> MERLFEELAGEAVKELLRAVRGTFFCRSTAERLRRNVEPLLPLVQPQAAQGGGGWGHGRSAGELAELAAQLREALELARRAASAPRWNVYRTAQLARRMEAADTAIARWLSRHAPAHVLDGVRRLRDEADARIGRLERRVEEVAAAQQQQQAAATALPPPAISLPFALPPPPPPPKAMAMMAMDTPPTKGMAVGMEVELPFPDDEEDESMVGGGVRVGKEKVKEMVMSGGGGGWEAVGICGMGGSGKTTLAMEIFKDHKIRGYFSDRVFFETISQSANLDTIKMKLWEQISGNLVLGAYNQIPEWQLKLGPRDKGPVLVILDDVWSLSQLEELIFKFPGCKTLVVSRFKFPSLVTR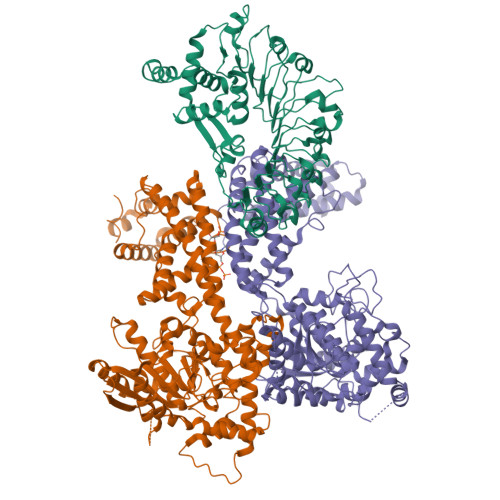TYEMELLDEEAALSVFCRAAFDQESVPRTADKKLVRQVAAECRGLPLALKVIGASLRDQPPKIWLSAKNRLSRGETISDSHETKLLERMAASIECLSGKVRECFLDLGCFPEDKKIPLDVLINIWMEIHDLDEPDAFAILVELSNKNLLTLVNDAQNKAGDLYSSYHDFSVTQHDVLRDLALHMSGRDALNNRRRLVMPRREESLPKDWQRNKDTPFEAQIVSIHTGEMKESDWFQMSFPKAEVLILNFASSVYYLPPFIATMQNLKALVLINYGTISATLDNLSAFTTLSDLRSLWLEKITLPPLPKTTIPLKNLRKISLVLCELTNSLRGSKVDLSMTFPRLSNLTIDHCIDLKELPSSICEISSLESISISNCHDLTELPYELGKLHCLSILRVYACPALWRLPPSVCSLKRLKYLDISQCVNLTDLPEELGHLTSLEKIDMRECSRLRSLPRSSSSLKSLGHVVCDEETALLWREAEQVIPDLRVQVAEECYNLDWLVD;> MPAAAALSDDDRLVVAHCAALSFPPASQPPPPPTTSSSSSGAGAGASFQVHHASHPYPCAAFAFPPSWSAAPGWAAAGRAAFGDAEVDPSLFPSLRSVGSGVPARANAAFLASFGALLDGSPLQSEVSRAVAEEKRIVFTGHSSGGSIATLAAIWFLETCTRRGSVNQAHPFCVTFGAPLVGDNTFNNAVRREGWSQCILNFVVPVDIIPRIPLTPLASATEGIQAVLDWLSPQTPNFSPSGMPLIISQFYENLLRSTLSIASYEACSFMGCTSSILGTLTSFIELSPYRPCGTYLFLTSSEQLAVLTNSDAVLQLLFYCLQLDPQQQLRDAAERSLSAHWQYEPIKQSMMQEIVCVDYLGVVSSTLPGRQMSSTIVGGLELSKEAMLSLSAAGQWEKQRETNQAKIDGASCTKIREALKSLNEYKRTCELHEVSYYDSFKLQREVHDFNANVSRLELAGLWDEIVEMLRRRELPDGFESRQDWVNLGTLYRRLVEPLDIANYYRHSKNEDTGSYLSKGRPRRYKYTQEWHEQSQRISFGSSLESCFWAMAEELQAEIANGKTFEDVRDRVVKLESDAHGWSMSGSLGKDIFLSRSSFVIWWKTLPENHRSASCIAKLVPW;> MEDASRGEEENSMFETSHVLGALLASSPLLARAWDRCAAAADGGASSLGFVHGGGGGGEGEPVCVAFSGVQAALSAAAGGGGGAEIFKPVGLRGDAAGRLFAPLVAAEPEDAGGEPVAVQALALQGFLRLCRSPEFQVLLNQIRGKAVVFTGHSLGGAIAALVALHYLCTSSSSSAFAPAPPVLCVTFGSPLLGNQALSRAILRERWAGNFCHVVSQHDVVPRLLFCPLNVIPVHIVVGMQLHQLPVRARRAAGVVATVTARMADTNQESLRQLIQEHAGEAAIEQKLAAPEIPSGSPYRPFGAYVLCSPDGAACVDNPTAAVQMLYATFAARRAPETGAVPPEAAHSCYGDLVLSMPHHLLLKRRLGATVTAPAASNYDVGISIALEASGITGEATEAAPARQWLKTSKRVGRSPSLNCASLATRLGRITPCRAQIEWYKALFDANTGYYDAFKQRLSPKKFSKANMYRIKLAQFWDGVLSMLDTSQLPYDFHRRAKWVNAAHFYQLLVEPLDIADYHRNNLHRTRGSYITHGRERRYELFDKWWKQKGCTDPSTGDTSATTTARRSKFAGLTQDPCFWARVEEAREQTESAKSERDMTSLARMLEDLHKFERHSSELVENKEVSIDVVAPQSSYSLWVKEWNELKLREEVRTILFQF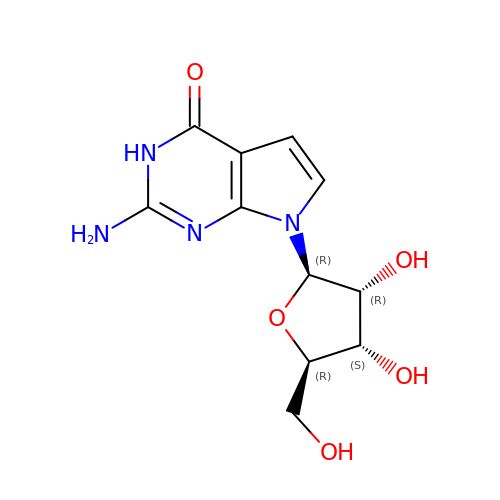2-azanyl-7-[(2R,3R,4S,5R)-5-(hydroxymethyl)-3,4-bis(oxidanyl)oxolan-2-yl]-3H-pyrrolo[2,3-d]pyrimidin-4-one | C11 H14 N4 O5 | JRYMOPZHXMVHTA-DAGMQNCNSA-N> MLESNENRIQIMSTIAKIY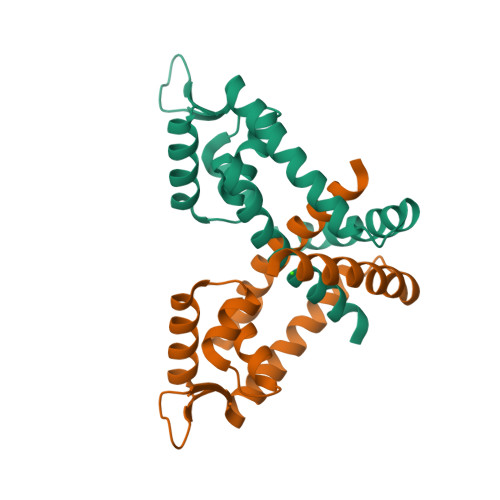RAMSRELNRRLGELNLSYLDFLVLRATSDGPKTMAYLANRYFVTQSAITASVDKLEEMGLVVRVRDREDRRKILIEITEKGLETFNKGIEIYKKLANEVTGDLSEDEVILVLDKISKILKRIEEISQ(4S)-N-{4-AMINO-5-[(2-AMINOETHYL)(HYDROXYAMINO]-PENTYL}-N'-NITROGUANIDINE | C8 H21 N7 O3 | 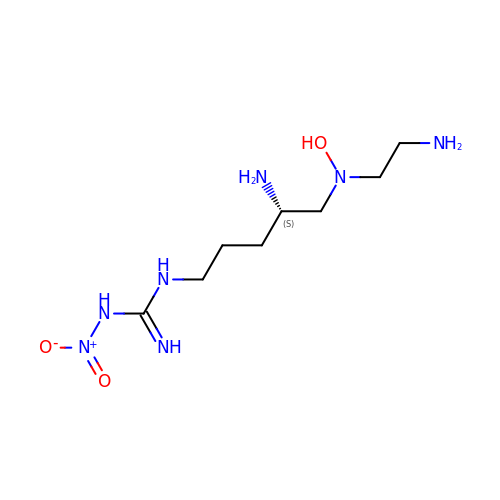HUOGRSGQHCPAGO-ZETCQYMHSA-N In this work, we selected CYP105A1 from Streptomyces griseolus to study the biochemical and structural mechanisms of inhibition. CYP105A1 can catalyze 2-step (25- and 1α-) hydroxylation reactions of vitamin D3 (VD3) to produce hormonally active 1α,25-dihydroxyvitamin D3 (1α,25(OH)2D3). The structures show that the ligand binding pocket is predominantly surrounded by hydrophobic residues, although there are three arginine residues (Arg73, Arg84, and Arg193) in the binding pocket. Our previous studies showed that wild-type and mutant CYP105A1 metabolize 12 types of non-steroidal anti-inflammatory drugs (NSAIDs), including diclofenac, with the R84A mutant exhibiting particularly high activity towards many NSAIDs.

Ketoconazole and miconazole clearly exhibited competitive inhibition, whereas lanoconazole exhibited noncompetitive inhibition. The Ki (inhibition constant) values for ketoconazole, lanoconazole, and miconazole calculated from their Dixon plots were 22.68 ± 2.33, 0.90 ± 0.10, and 1.20 ± 0.35 μM. The structures of the EI complexes show that ketoconazole binds to the heme iron in a single conformation, whereas lanoconazole and miconazole each bind in two conformations. Thus, the allowed conformation of ketoconazole for binding to the heme in the binding pocket is highly restricted compared with those of lanoconazole and miconazole. In the ketoconazole complex, one chloride of the dichlorophenyl group is positioned 3.35 Å from the side chain Nη2 of Arg73 and 3.46 Å from a water molecule, and the oxygen of the terminal acetyl group is 3.60 Å and 3.29 Å from the side-chain hydroxyl oxygens of Thr81 and Ser82, respectively. The terminal residues of the F helix and the residues in the F-G loop are positioned differently in the ketoconazole complex compared with the lanoconazole and miconazole complexes due to the phenyl group of ketoconazole being located near Val181 in the F helix. The position of the I helix is similar amongst the EI complexes, but His246 is flipped in the ketoconazole complex. In addition, the binding pocket must undergo structural changes to accommodate ketoconazole, including positional changes of the F helix and in His246 and surrounding residues. The structural properties of ketoconazole show that the entropic cost of binding to the heme is larger for ketoconazole than for lanoconazole and miconazole. Therefore, ketoconazole showed a lower affinity (larger Kd value) than the other two inhibitors.

> MTDTATTPQTTDAPAFPSNRSCPYQLPDGYAQLRDTPGPLHRVTLYDGRQAWVVTKHEAARKLLGDPRLSSNRTDDNFPATSPAFEAVRESPQAFIGLDPPEHGTRRRMTISEFTVKRIKGMRPEVEEVVHGFLDEMLAAGPTADLVSQFALPVPSMVICRLLGVPYADHEFFQDASKRLVQSTDAQSALTARNDLAGYLDGLITQFQTEPGAGLVGALVADQLANGEIDREELISTAMLLLIAGHETTASMTSLSVITLLDHPEQYAALRADRSLVPGAVEELLRYLAIADIAGGRVATADIEVEGQLIRAGEGVIVVNSIANRDGTVYEDPDALDIHRSARHHLAFGFGVHQCLGQNLARLELEVILNALMDRVPTLRLAVPVEQLVLRPGTTIQGVNELPVTWHHHHHH The bifunctional enzyme Δ1-pyrroline-5-carboxylate synthase (P5CS) is vital to the synthesis of proline and ornithine, playing an essential role in human health and agriculture. The P5CS molecule contains two domains, GK and GPR, catalyzing the first and second steps in the biosynthesis of proline from glutamate. The GK domain catalyzes glutamate phosphorylation, and the GPR domain catalyzes the NADPH-dependent reduction of γ-glutamyl phosphate (G5P) to glutamate-γ-semialdehyde (GSA). Our results describe the assembly mechanism of P5CS filaments, in which the GK domain forms tetramer and the GPR domain forms dimer structure, and both domains form specific interaction interfaces.

In the P5CSGlu/ATPγS filament, the ligands could not be determined due to incomplete densities. The GK domain structure of the P5CSGlu/ATPγS filament is virtually identical to that of the P5CSMix filament. We speculate that there are two ligand-binding modes (bound with Glu-Mg-ATPγS and G5P-Mg-ADP, respectively) in the P5CSGlu/ATPγS filament. These two modes may coexist in the active sites of the GK tetramer, thereby affecting the 3D reconstruction of the structures. The unexpected presence of G5P could be due to the contamination of ATP in the commercial ATPγS (80% pure) and all substrates were in excess during our sample preparation. Thus, no ligand was modeled in the GK domain structure of the P5CSGlu/ATPγS filament. In P5CSGlu/ATPγS and P5CSMix filaments, the additional interface between hook structures pairs locks adjacent GK tetramers.

>[2x]MLQNSFKLAQSLRNGFYRNAWRAFSSHGPRQPLVSPERRLEKAHPTFTERSQLKYARRLVVKLGSAVITREDNHGLALGRLASIVEQVAECHLEGREVMMVTSGAVAFGKQKLAQELLMSLSMRETLNPKDSKEFDGATLEPRAAAAVGQSGLMSLYDAMFAQYGVKIAQVLVTKPDFYNEETRNNLFCTLSELISLNIVPIINTNDAVSPPMFIRDDEPAGGARRGIPIKDNDSLSAMLAAEVQADLLILMSDVDGIYNKPPWEDGAKLMHTYTSDDSNSIEFGKKSKVGTGGMDSKVKAATWALDRGVSVVICNGMQEKAIKTIIGGRKVGTFFTEATESANAVPVEVMAENARTGSRQMQALTPAQRASAVNTLADLLVSREKFILDANAKDLAEAQKSGLAKPLLSRLSLNPAKLKNLSVGLKQIAEDSHKNVGRVLRRTRLADQLELKQVTVPIGVLLVIFESRPDSLPQVAALAMASANGLLLKGGKEAAHSNKALMELVKEALATVGAEHAVSLVSTREEISDLLSMENHIDLIIPRGSSDLVRSIQQQSLHIPVLGHAEGVCHVYIDRDADLEKALRIARDAKCDYPAACNAMETLLIHEDLMSGAIFGDVCNMLKREGVKIYAGPRLNQQLTFGPPAAKSLKHEYGALECCIEVVPSLDEAINHIHTYGSSHTDVIVTENDAAARQFLGSVDSACVFHNASSRFADGFRFGLGAEVGISTARIHARGPVGVEGLLTTKWILEGQDHAAADFAEGGGRTWLHETLPLD> SMGNLIKVLTRDIDHNASHFFLDFENAQPTEAEREIFNQVNVVLKDAEGILNDLQSYRGAGHEIREAIQHPNDENLQEKAWSAVCPLVGKLKKFYEFSQRLEAALHGLLGALTSTPYSPTQHLEREQALAKQFAEILHFTLRFDELKMTNPAIQNDFSYYRRTLSRMRINNVPAEGENEVNNELANRMSLFYAEATPMLKTLSDATTKFVSDNK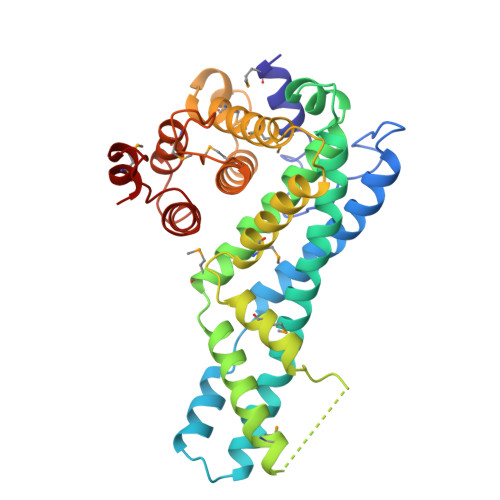SLPIENTTDCLSTMASVCRVMLETPEYRSRFASEETVSFCLRVMVGVIILYDHVHPVGAFAKTSKIDMKGCIKVLKDQPPNSVEGLLNALRYTTKHLNDETTSKQIKTMLQ> SSASAAAAAAAAALAAGAADGPTNDEAPGADGRRSYINLPAHHSAIIQQWVLDAGSGSILGHVNGGFLPNPVAAHSGSEFALASTSFSRIAKGKRTDYVEVFDPVTFLPIADIELPDAPRFDVGPYSWMNANTPNNADLLFFQFAAGPAVGLVVQGGSSDDQLLSSPTCYHIHPGAPSTFYLLCAQGGLAKTDHAGGAAGAGLVGAMLTAAQNLLTQPAQANKSGRIVWPVYSGKILQADISAAG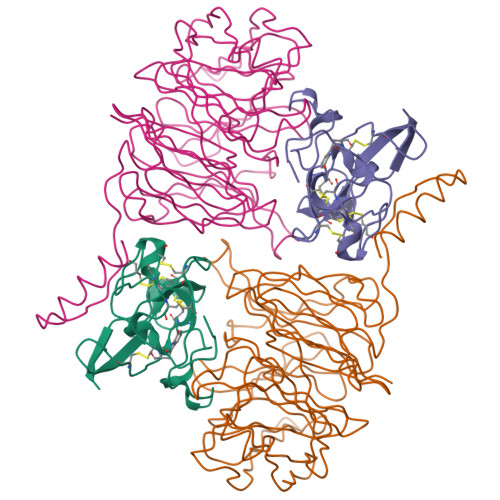ATNKAPIDALSGGRKADTWRPGGWQQVAYLKSSDGIYLLTSEQSAWKLHAAAKEVTSVTGLVGQTSSQISLGHDVDAISVAQDGGPDLYALSAGTEVLHIYDAGAGDQDQSTVELGSGPQVLSVMNEA;> VDPRAKWQPQDNDIQACDYWRHCSIDGNICDCSGGSLTNCPPGTKLATASWVASCYNPTDGQSYLIAYRDCCGYNVSGRCPCLNTEGELPVYRPEFANDIIWCFGAEDDAMTYHCTISPIVGKA>MHFVHMRGLPFQANAQDIINFFAPLKPVRITMEYSSSGKATGEADVHFETHEDAVAAMLKDRSHVHHRY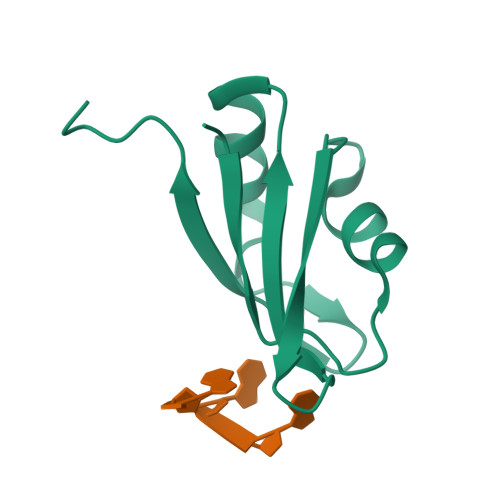IELFLNSCPKGK[4x]(4-pyrimidin-5-ylphenyl)methanol | C11 H10 N2 O | 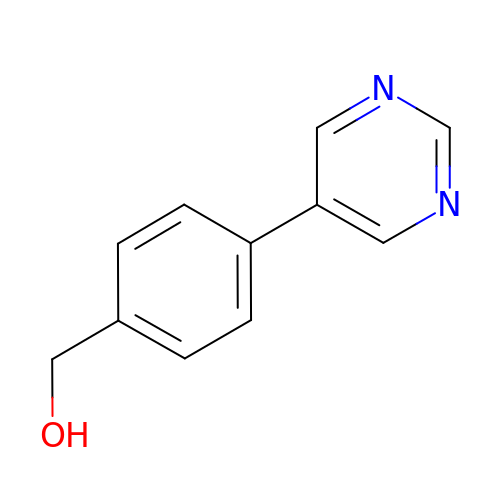QPOIDCHBWLGFGU-UHFFFAOYSA-N Sterol 14α-demethylase (CYP51) is the cytochrome P450 that removes the 14α-methyl group from the sterol core. The molecular evolution of cytochromes P450 and associated redox-driven oxidative catalysis remains a mystery in biology. It is widely believed that sterol 14α-demethylase (CYP51), an essential enzyme of sterol biosynthesis, is the ancestor of the whole P450 superfamily given its conservation across species in different biological kingdoms. Herein we have utilized X-ray crystallography, molecular dynamics simulations, phylogenetics and electron transfer measurements to interrogate the nature of P450-redox partner binding using the naturally occurring fusion protein, CYP51-ferredoxin found in the sterol-producing bacterium Methylococcus capsulatus. Our data advocates that the electron transfer mechanics in the M. capsulatus CYP51-ferredoxin fusion protein involves an ensemble of ferredoxin molecules in various orientations and the interactions are transient.

The lanosterol-bound M. capsulatus CYP51-fx fusion protein was crystallized in the P1211 space group, and the structure was resolved to 2.5 Å resolution. The asymmetric unit consisted of four molecules of P450, the active site of each containing one molecule of lanosterol. In all the three structures the sterol 14α-methyl group lies within 4.1–4.2 Å from the heme iron, i.e., they are clearly captured in the catalytically competent orientation. Firstly, there is an additional H-bond between the sterol C3-OH and the side chain OH of Y186 (located in helix F’’) not seen in eukaryotic CYP51s. This bond strongly implies that M. capsulatus CYP51 binds sterol substrates with higher affinity than its corresponding eukaryotic orthologs. A second unique feature of the M. capsulatus CYP51 structure is that binding of the substrate does not free the side chain of E178 (helix F) from a salt bridge, an event essential to activate proton delivery in the eukaryotic CYP51 orthologs. Although the H-bond with the CYP51 family signature histidine (the residue preceding the conserved P450 threonine in the I helix, H260 in M. capsulatus) is lost, a new and stronger salt bridge (2.8 Å) is now formed between the E178 hydroxyl and the neighboring H259 (this residue is unique and highly conserved in bacterial CYP51s15). This indicates that, in contrast with the eukaryotic CYP51s structures, the presence of the substrate alone does not complete switching the M. capsulatus CYP51 domain to an active conformation. Despite these readjustments, however, the electron density for the ferredoxin domain (or even the [2Fe-2S] cluster) in the structure of the fusion protein was still absent. Upon binding of the substrate all these three residues were shown to lose their contact with the heme, the side chain flipping up towards the proximal P450 surface and playing a role in the ET process.

>MSHPPSNTPPVKPGGLPLLGHILEFGKNPHAFLMALRHEFGDVAEFRMFHQRMVLLTGSQASEAFYRAPDEVLDQGPAYRIMTPIFGRGVVFDARIERKNQQLQMLMPALRDKPMRTYSEIIVAEVEAMLRDWKDAGTIDLLELTKELTIYTSSHCLLGAEFRHELNTEFAGIYRDLEMGIQPIAYVFPNLPLPVFKRRDQARVRLQELVTQIMERRARSQERSTNVFQMLIDASYDDGSKLTPHEITGMLIATIFAGHHTSSGTTAWVLIELLRRPEYLRRVRAEIDALFETHGRVTFESLRQMPQLENVIKEVLRLHPPLILLMRKVMKDFEVQGMRIEAGKFVCAAPSVTHRIPELFPNPELFDPDRYTPERAEDKDLYGWQAFGGGRHKCSGNAFAMFQIKAIVCVLLRNYEFELAAAPESYRDDYRKMVVEPASPCLIRYRRRDAPAAVDAKASAGEAPAETLRGAFRVTVDRDLCKGHGNCMAEAPEIFRVDEDGRLTLLSETPDPVLVGAALAAERFCPARAIKILPQRDPATRDRSLSPSGED[4x]>[2x]GAMASHMTEIALIGNPNSGKTSLFNLITGHNQRVGNWPGVTVERKSGLVKKNKDLEIQDLPGIYSMSPYSPEAKVARDYLLSQRADSILNVVDATNLERNLYLTTQLIETGIPVTIALNMIDVLDGQGKKINVDKLSYHLGVPVVATSALKQTGV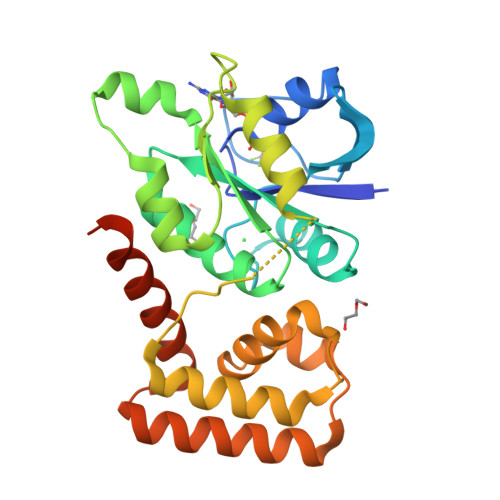DQVVKKAAHTTTSTVGDLAFPIYDDRLEAAISQILEVLGNSVPQRSARFYAIKLFEQDSLVEAELDLSQFQRKEIEDIIRITEEIFTEDAESIVINERYAFIERVCQMAESHTEDFALTLS> MENLYFQGAKIGLFYGTQTGVTQTIAESIQQEFGGESIV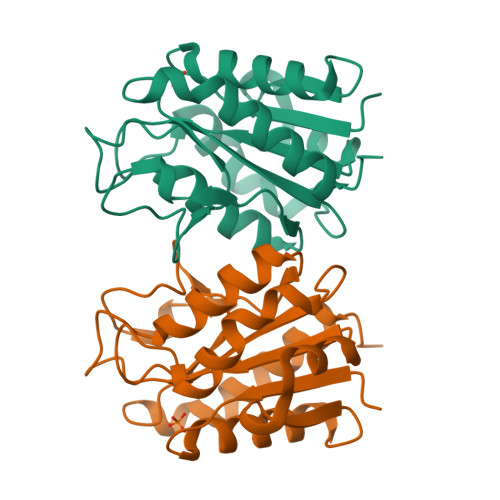DLNDIANADASDLNAYDYLIIGCPTWNVGELQSDWEGIYDDLDSVNFQGKKVAYFGAGDQVGYSDNFQDAMGILEEKISSLGSQTVGYWPIEGYDFNESKAVRNNQFVGLAIDEDNQPDLTKNRIKTWVSQLKSEFGLALEHHHHHH> S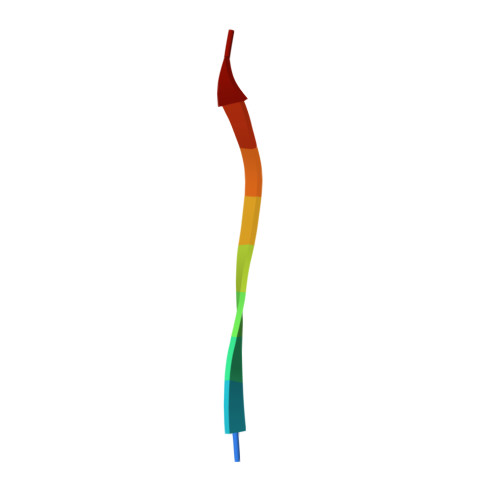RIRIRGYVR>[4x]SNAEEAENDLTQLANKVAVILENHEDQALARSITWELA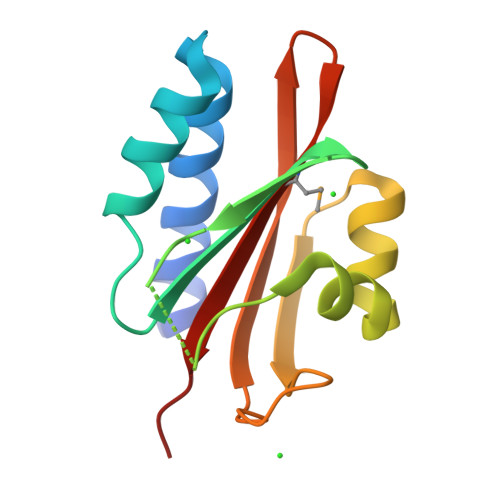DNLTSIAIIQDEKNHWYSPNDKNRLSSITVEQIQHDKDLNKALKDHKKVSKRTGLSDTDTDNERLIVGVPYEKDGKKGMVFLSQSLLA>[6x]MATLATKKATLVAALK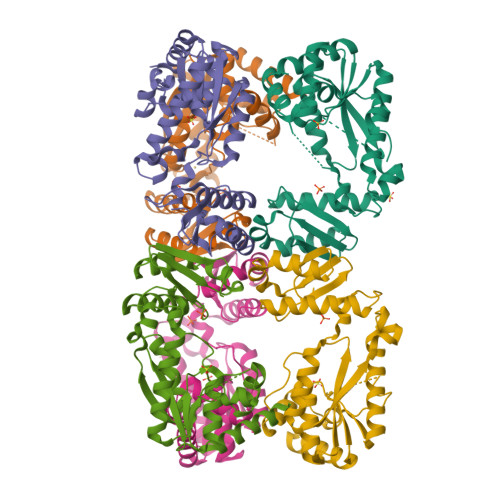DLQRVTVAFSGGIDSTLVLKMALDVLGRDNVTAVVANSELFTDEEFDKAMSLAEELGANVQGTTLDYLSDDHIKNNTPDSWYYAKKMFYSRLNDIAANNGSAAVLDGMIKNDENDYRPGLKARSEAGARSLLQEADFFKTDVRALAQELGLTNWNKVASCSVSSRFPYGTTLTHDNIAQVMAAEKYLRSLGFPTVRVRFHNDIARIELPEARIGDFLVFNDRVNRQLQSLGFRYVTLDLGGFRSGRMNDTLTKAQLATFAASWSHPQFEK>GSQEEDLPRPSISAEPGTVIPLGSHVTFVCRGPVGVQTFRLERESRSTYNDTEDVSQASPSESEARFRIDSVSEGNAGPYRCIYYKPPKWSEQSDYLELLVKEAAA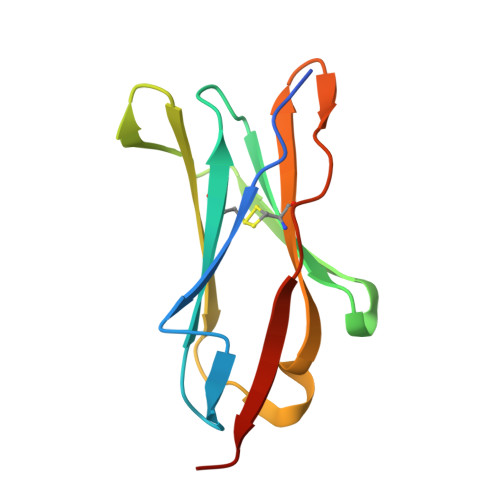[3x]>HPETLVKVKDAEDQLGARVGYIELDLNSGKILESFRPEERFPMMSTFKVLLCGAVLSRIDAGQEQLGRRIHYSQNDLVAASPVTEKHLTDGMTVRELCSAAITMSDNTAANLLLTTIGGPKELTAFLHNMGDHVTRLDRWEPELNEAIPNDERDTTMPAAMATTLRKLLTGELLTLASRQQLIDWMEADKVAGPLLRSALPAGWFIADKSGAGERGSRGIIAALGPDGKPSRIVVIYTTGSQATMDERNRQIAEIGASLIKHW[2x];>[2x]AGVMTGAKFTQIQFGMTRQQVLDIAGAENCETGGSFGDSIHCRGHAAGDYYAYATFGFTSAAADAKVDSKSQEALLAPSAPTLTLAKFNQVTVGMTRAQVLATVGQGSCTTWSEYYPAYPSTAGVTLSLSCFD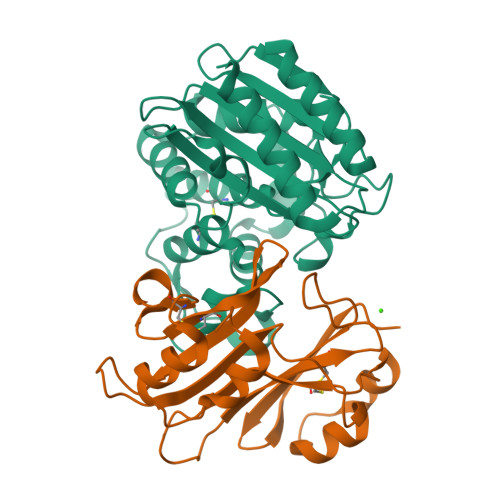VDGYSSTGAARGSAHLWFTDGVLQGKRQWDLV> AEPDHPIQLVWTDVNGRLSLDLSGAHDCFLNTRYSNYPVFILCIIGEKRRGKSFLMNYIMRALRSMEMDEEISLGADDEPLKGFKWSPGTETTTKGIWMWNRPFLLNHKGGKIAVFLLDTEGSLDIESDRETCIKLSALSLFISSHLIFNVASNLKETELDYMEMYMNMGEECGPKNLQHLDILVRDWYHSKKWDRDVARSYISREIEKLEKLNSYPKVLWSLKSNQTRCFLLPHPGKGITGESEGRLQDMDE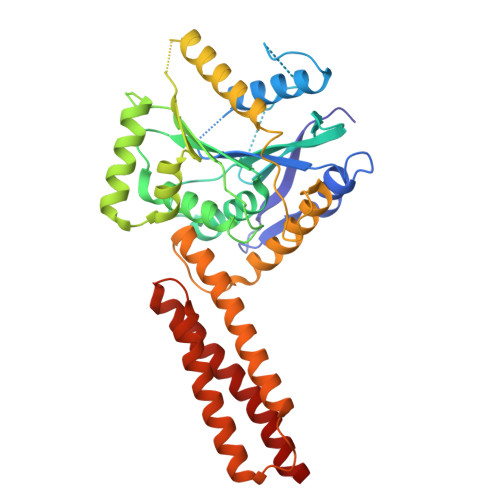DFQESLRSYVSKVVKGICTHIKTNIDGELLTSAHVFSMLQEFTEVLNLQIYGFSSPMEMFYAIKNQKLMGEIENEFQDFLKNQSSLTLPPTMRVKVSQKFSELLEKFMQFVQGSNTSSHDAMLKDLEVRLLEIQEKFCNDFTTRFT> NAMKCWSSSCFWKKASNGLVVIPYVISSEYSGGEVATIEGAMRAFNGKTCIRFVRRTN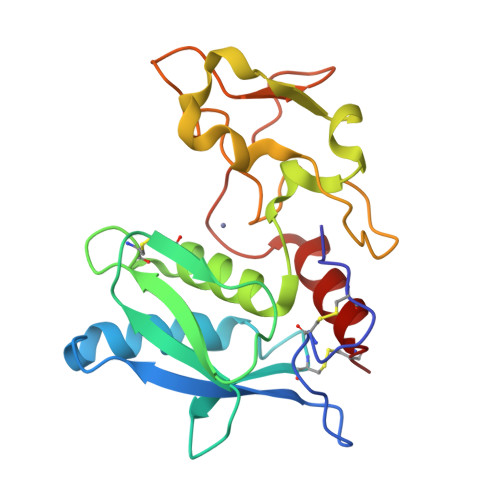EYDFISVVSKTGCYSELGRKGGQQELSINRGGCMYSGIIQHELNHALGFQHEQTRSDRDSYVRINWENIIPASAYNFNKHDTNNLNTPYDYSSIMHYGRDAFSIAYGRDSITPIPNPNVPIGQRNGMSRWDITRINVLYNCR>GYTLWNDQIVKDEEVKIDKEDRGYQFGDGVYEVVKVYNGEMFTVNEHIDRLYASAEKIRITIPYTKDKFHQLLHELVEKNELNTGHIYFQVTRGTSPRAHQFPENTVKPVIIGYTKENPRPLENLEKGVKATFVEDIRWLRCDIKSLNLLGAVLAKQEAHEKGCYEAILHRNNTVTEGS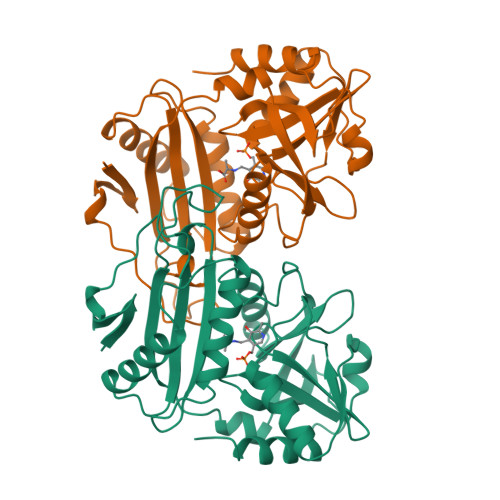SSNVFGIKDGILYTHPANNMILKGITRDVVIACANEINMPVKEIPFTTHEALKMDELFVTSTTSEITPVIEIDGKLIRDGKVGEWTRKLQKQFETKIP[2x]>M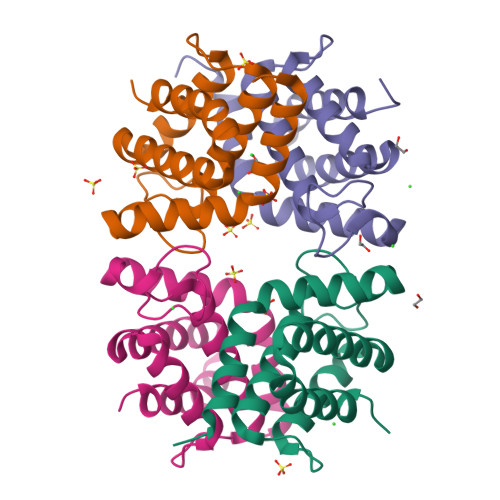KTSEQRVNIATLLTENKKKIVDKASQDLWRRHPDLIAPGGIAFSQRDRALCLRDFGWFLHLITFCLLAGDKGPIESIGLISIREMYNSLGVPVPAMMESIRCLKEASLSLLDEEDANETAPYFDYIIKAMSHHHHHH[4x]> MGGSHHHHHHGENLYFQSVDDLTVEPNLHSLITSTTHKWIFVGGKGGVGKTTSSCSIAIQMALSQPNKQFLLISTDPAHNLSDAFGEKFGKDARKVTGMNNLSCMEIDPSAALKDMNDMAVSRANNNGSDGQGDDLGSLLQGGALADLTGSIPGIDEALSFMEVMKHIKRQEQGEGETFDTVIFDTAPTGHTLRFLQLPNTLSKLLEKFGEITNKLGPMLNSFMGAGNVDISGKLNELKANVETIRQQFTDPDLTTFVCVCISEFLSLYETERLIQELISYDMDVNSIIVNQLLFAENDQEHNCKRCQARWKMQKKYLDQIDELYEDFHVVKMPLCAGEIR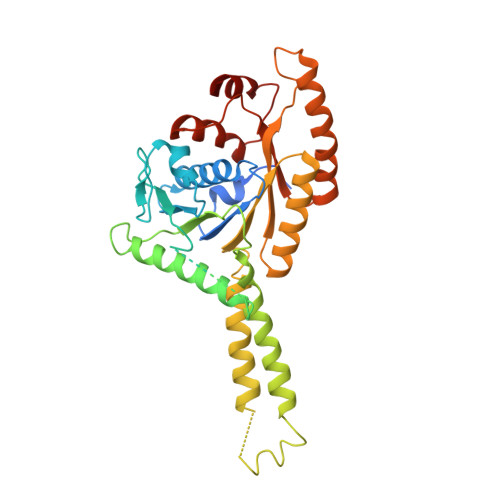GLNNLTKFSQFLNKEYNPITDGKVIYELEDKE> MIRVLFFIRMTMSRTIQRICLFLFCLPVFGSCMKWDYGEMEDFSVSASGLFITNEGNFQYSNATLSYYDPATCEVENEVFYRANGFKLGDVAQSMVIRDGIGWIVVNNSHVIFAIDINTFKEVGRITGFTSPRYIHFLSDEKAYVTQIWDYRIFIINPKTYEITGYIECPDMDMESGSTEQMVQYGKYVYVNCWSYQNRILKIDTETDKVVDELTIGIQPTSLVMDKYNKMWTITDGGYEGSPYGYEAPSLYRIDAETFTVEKQFKFKLGDWPSEVQLNGTRDTLYWINNDIWRMPVEADRVPVRPFLEFRDTKYYG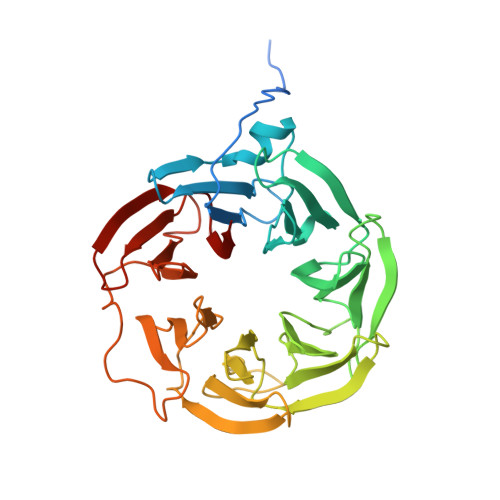LTVNPNNGEVYVADAIDYQQQGIVYRYSPQGKLIDEFYVGIIPGAFCWK>[12x]MLYTDSLNYKQLSTVSDDMQSYLPVAKEIAKIAQGGHELDPEDYLLIRDEESPGVTKKRIEKFAPENYLGAAIRLQRVLQKSGVLEIKSDSLPGDLTVWESFFNKVDKRNSSLKDFVIDVFTEALVNKYCYVQVELSKLDFDTVTEAEAEGILSTRKPYYFKIPLQSIMVEKCDGDTIQWIKYKRLDKIDNPFDKTIYNMSYVLIDDQHITTWTYYDIIVSDSGG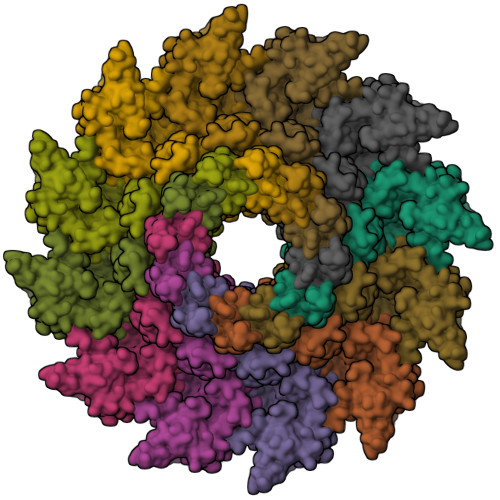ISKIWDQSLNYGKGAYRSIDKEKDKADPVSFAHNRGSCPVVRYRMDESLYMADQVYLAQRMIYGLSMNLFHTAANAGFVQKWIRPYIAGNDTRISKESGGASYIPLPKEALNEIIKKYAESLGDESVIMADFFTFEELAGTSVEMQIGLIERLRNYIFTAILFNNAKFEQSTSDSQSGAAKEIDFYVQNLALKDHGSGIVEFTRSLLHHTAKAFGYDSGGSIVVSGMDRYDVRPIEQVLSLIERLFKLPQLAIPKDLLIESMSQLSRLIIENTTFEYKNTLNDAIISNIDEYLNSVKKQSNDAFNETVK> HMKSVFVESTIFEKYRDEYLSDEEYRLFQAELMLNPKLGDVIQGTGGLRKIRVASKGKGK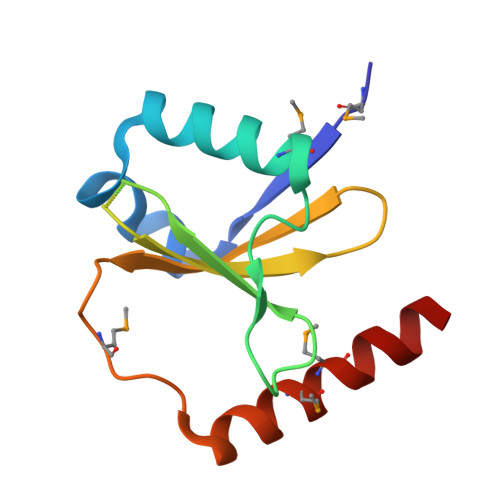RGGSRIIYYFLDEKRRFYLLTIYGKNEMSDLNANQRKQLMAFMEAWRNEQS Some Gram-negative bacteria target their competitors by exploiting the type VI secretion system to extrude toxic effector proteins. To prevent self-harm, these bacteria also produce highly specific immunity proteins that neutralize these antagonistic effectors. The opportunistic pathogen Serratia marcescens has recently been shown to utilize T6-dependent secretion of two family 4 amidases, Ssp1 and Ssp2, to mediate antibacterial activity. In S. marcescens, the resistance-associated proteins Rap1a and Rap2a neutralize Ssp1 and Ssp2, respectively.

Established functional assays were utilized to examine the effect of mutating the catalytic cysteine (Cys50) of Ssp1 and Ssp2. Isomorphous crystal structures of Ssp1 (at 1.85 Å resolution) and the active-site Ssp1-C50A mutant (at 2.2 Å resolution) reveal the overall enzyme structure and details of the active site. The protein is a monomer in solution but crystallized with two molecules in the asymmetric unit, each consisting of residues 1–163. The root-mean-square deviations (r.m.s.d.s) between least-squares superimposed Cα atoms gives an average of 0.3 Å when comparing the four polypeptides in the crystal structures. The copies in the asymmetric unit are therefore judged to be essentially identical and neither mutagenesis of the catalytic Cys50 nor crystal lattice packing interactions induces any major structural changes. We conclude that mutation of the catalytic cysteine in Ssp1 and Ssp2 abolishes their bacteriolytic effect because the dl-endopeptidase activity is compromised. Furthermore, we can conclude that the Ssp–Rap interaction does not depend on the catalytic cysteine and that recognition of the Ssp effectors by the T6SS machinery is also independent of their enzymatic activity.

>[2x]MKPLYRQLKSSHYSSDYSSPGYLAAEAVYAEIGYELDTLLKQNPGYANTAAVRMSLALLKTGISFKGRLPIKKGAYKGKTIEPGAKLLADQLHRSSSFGKAKIFFNAPDAEKGIGNKKGVVFFNKITNYDGGHIDLIEPENSLLTCHSHCYFNCKEVWFWELS> MAVKIKIEHLTKIFGKRIKTALTMVEKGEPKNEILKKTGATVGVYDTNFEINEGEIFVIMGLSGSGKSTLLRLLNRLIEPTSGKIFIDNQDVATLNKEDLLQVRRKTMSMVFQNFGLFPHRTILENTEYGLEVQNVPKEERRKRAEKALDNANLLDFKDQYPKQLSGGMQQRVGLARALANDPEILLMDQAFSALDPLIRREMQDELLELQAKFQKTIIFVSHDLNEALRIGDRIAIMKDGKIMQIGTGEEI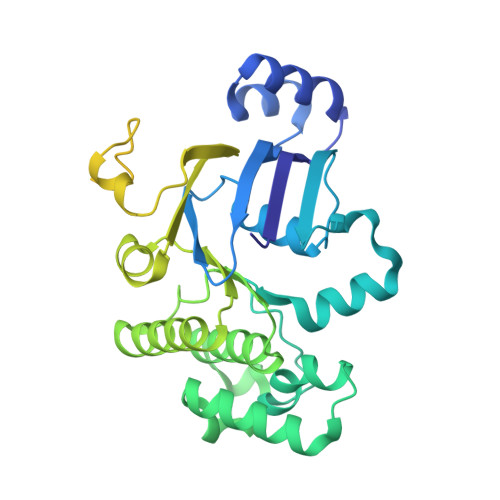LTNPANDYVKTFVEDVDRAKVITAENIMIPALTTNIDVDGPSVALKKMKTEEVSSLMAVDKKRQFRGVVTSEQAIAARKNNQPLKDVMTTDVGTVSKEMLVRDILPIIYDAPTPLAVVDDNGFLKGVLIRGSVLEALADIPDEDEVEEIEKEEENK>[2x]MMTNLETRLSGADPVFARELHAQLVQALGDVKRRLLRGGTQQQYQQWQQEADAIEAGLNIIEKIKGE;>MNVQLKKQLAELALAGTGHHCHQEAASIADWLAQEECMAECVTLIRLSSLMNQGDYQRALL[2x]

Many Gram-negative bacteria exploit host cellular functions through the use of type III secretion systems (T3SSs) for host penetration and effector delivery. Chaperone proteins are required to avoid premature oligomerization of the needle complex subunit or translocators, and to maintain effectors in a form ready to be translocated in the T3SS system. The class III chaperone for the needle complex subunit is unique in that it is a heterodimer comprising E and G proteins. Although the N-terminal 14 residues of AscE may not be required to complex with G and F, AscE itself is essential to keep AscG soluble, monomeric, stable and with a disordered region to interact with AscF.

Here, we report the crystal structure of the ordered AscG1–61 region in complex with AscE at 2.4 Å resolution. Each asymmetric unit contained two molecules of AscE-AscG1–61 complex. The helices α2 (residues 14–35) and α3 (residues 44–65) of AscE formed a pair of anti-parallel helices in the AscE-AscG1–61 complex with a topology similar to those in the crystal structure of apo AscE. In contrast, when in complex with AscG1–61, this region was induced to form a two-turn helix, α1 (residues 4–12), located in a perpendicular orientation to α2, similar to that which is observed by PscE in the PscE-PscF-PscG complex. Here, we showed that the structure of AscG1–61 in the AscE-AscG1–61 complex consisted of an anti-parallel three helices bundle, with topology similar to the first on-and-a-half of the N-terminal TPR of PscG/YscG in both PscE-PscF-PscG/YscE-YscF-YscG complexes. Furthermore, in the AscE-AscG1–61 complex, only residues from the first TPR (αA, residues 3–20; and αB, residues 22–35) interacted with AscE, whereas the helix αC (residues 39–52) from the N-terminal half of the second TPR showed no points of contact with AscE. AscE residues Leu5 and Leu9 on helix α1; Leu20 and Leu24 on helix α2; and Ile54, Ile60, Ile61 and Ile64 on helix α3 formed a hydrophobic core between AscE and AscG1–61 through their interaction with AscG1–61. Leu5, Leu9 and Leu12 from helix αA, and Ile28 and Trp31 from helix αB of AscG1–61 were involved in forming the hydrophobic core with AscE. We identified that superposition of AscE-AscG1–61 had a rmsd of 1.1 Å with either PscE-PscF-PscG or YscE-YscF-YscG, suggesting that the orientation of AscE relative to AscG lies intermediate between PscE-PscF-PscG and YscE-YscF-YscG. Taking into consideration previous work in the field, we propose that AscE is required to keep the N-terminal region of AscG in a stable and ordered conformation, while the disordered C-terminal region of AscG will only be induced to fold upon interaction with the AscF substrate.> MILDTDYITEDGKPVIRIFKKENGEFKIDYDRNFEPYIYALLKDDSAIEDVKKITAERHGTTVRVVRAEKVKKKFLGRPIEVWKLYFTHPQDVPAIRDKIKEHPAVVDIYEYDIPFAKRYLIDKGLIPMEGDEELKMLAFDIETLYHEGEEFAEGPILMISYADEEGARVITWKNIDLPYVDVVSTEKEMIKRFLKVVKEKDPDVLITYNGDNFDFAYLKKRSEKLGVKFILGREGSEPKIQRMGDRFAVEVKGRIHFDLYPVIRRTINLPTYTLEAVYEAIFGQPKEKVYAEEIAQAWETGEGLERVARYSMEDAKVTYELGKEFFPMEAQLSRLVGQSLWDVSRSSTGNLVEWFLLRKAYERNELAPNKPDERELARRRESYAGGYVKEPERGL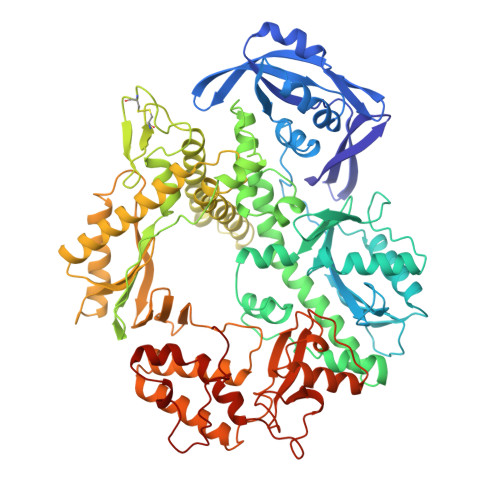WENIVYLDFRSLYPSIIITHNVSPDTLNREGCEEYDVAPQVGHKFCKDFPGFIPSLLGDLLEERQKVKKKMKATIDPIEKKLLDYRQRAIKILANSFYGYYGYAKARWYCKECAESVTAWGRQYIETTIREIEEKFGFKVLYADTDGFFATIPGADAETVKKKAKEFLDYINAKLPGLLELEYEGFYKRGFFVTKKKYAVIDEEDKITTRGLEIVRRDWSEIAKETQARVLEAILKHGDVEEAVRIVKEVTEKLSKYEVPPEKLVIYEQITRDLKDYKATGPHVAVAKRLAARGIKIRPGTVISYIVLKGSGRIGDRAIPFDEFDPAKHKYDAEYYIENQVLPAVERILRAFGYRKEDLRYQKTRQVGLGAWLKPKT>[12x]MMIRGIRGATTVERDTEEEILQKT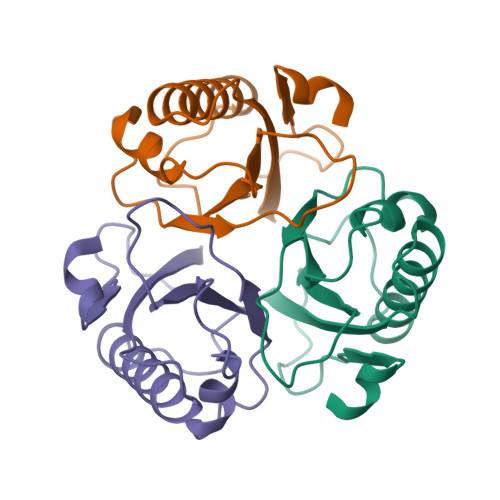KQLLEKIIEENHTKPEDVVQMLLSATPDLHAVFPAKAVRELSGWQYVPVTCMQEMDVTGGLKKCIRVMMTVQTDVPQDQIRHVYLEKAVVLRPDLSLTKNTEL>MVMSRLEGKIAIVTGASSGIGRAAALLFAREGAKVVVTARNGNALAELTDEIAGGGGEAAALAGDVGDEALHEALVELAVRRFGGLDTAFNNAGALGAMGEISSLSVEGWR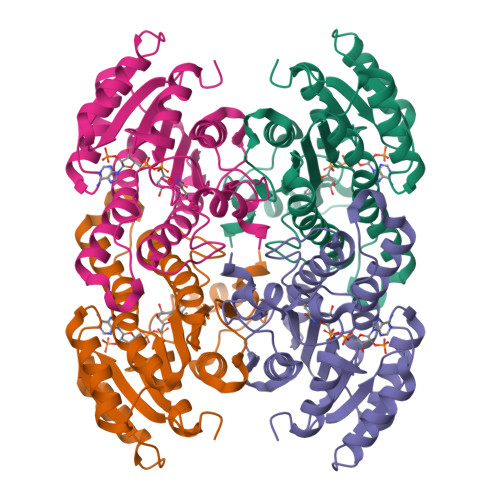ETLDTNLTSAFLAAKYQVPAIAALGGGSLTFTSSFVGHTAGFAGVAPYAASKAGLIGLVQALAVELGARGIRVNALLPGGTDTPANFANLPGAAPETRGFVEGLHALKRIARPEEIAEAALYLASDGASFVTGAALLADGGASVTKAAENLYFQSHHHHHHWSHPQFEK[8x]> MKTEWPELVGKGVAAAKKVILQDKPEAQIIVLPVGTIVTMEYRIDRVRLFVDKLDNIA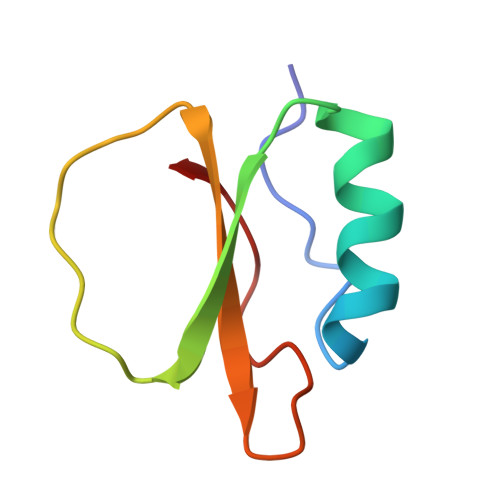QVPRVG>GPAMATNGEIFNTYGHNHQSATVTKITASNESSNG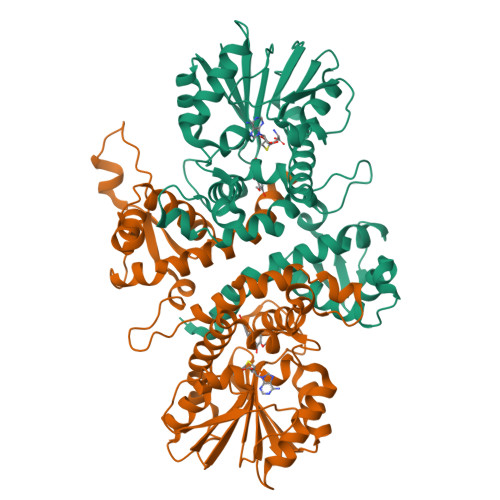VCYLSETANLGKLICIPMALRAAMELNVFQLISKFGTDAKVSASEIASKMPNAKNNPEAAMYLDRILRLLGASSILSVSTTAASINRGGDDVVVHEKLYGLTNSSCCLVPRQEDGVSLVEELLFTSDKVVVDSFFKLKCVVEEKDSVPFEVAHGAKIFEYAATEPRMNQVFNDGMAVFSIVVFEAVFRVYDGFLDMKELLDVGGGIGTSVSKIVAKYPLIRGVNFDLPHVISVAPQYPGVEHVAGDMFEEVPKGQNMLLKWVLHAWGDERCVKLLKNCWNSLPVGGKVLIIEFVLPNELGNNAESFNALIPDLLLMALNPGGKERTISEYDDLGKAAGFIKTIPIPISNGLHVIEFHK[2x]>[2x]GHMDLKTAVFNAARDGKLRLLTKLLASKSKEEVSSLISEKTNGATPLLMAARYGHLDMVEFLLEQCSASIEVGGSVNFDGETIEGAPPLWAASAAGHLKVVQSLLNHGASVNNTTLTNSTPLRAACFDGHLEIVKYLVEHKADLEVSNRH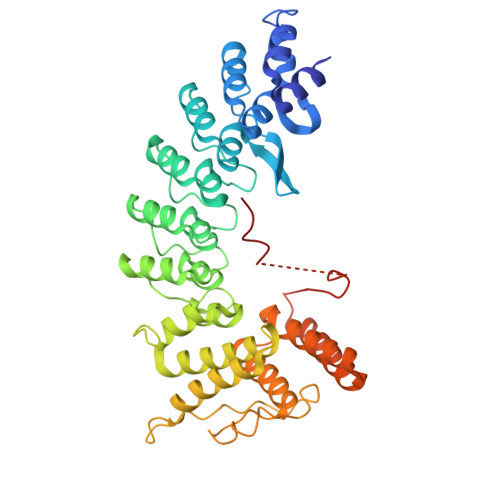GHTCLMISCYKGHKEIAQYLLEKGADVNRKSVKGNTALHDCAESGSLDIMKMLLMYCAKMEKDGYGMTPLLSASVTGHTNIVDFLTHHAQTSKTERINALELLGATFVDKKRDLLGALKYWKKAMNMRYSDRTNIISKPVPQTLIMAYDYAKEVNSAEELEGLIADPDEMRMQALLIRERILGPSHPDTSYYIRYRGAVYADSGNFKRCINLWKYALDMQQSNLDPLSPMTASSLLSFAELFGGGSGGGSGGGSGGGSSVNSLLKELR> MHRFRVCALGAAFCVARRWRSGGGPGDRRVRTDWYRCYPSLMEEKDRDMYHCYYPYLFDHGDKMSLYPKIPDNPREWQVEQLQTTYDAIREDKYDAFVRLRAKFPELYQDTYAWDNPPPFGEFNMFYSVRFGMIGVKAFTCKDYDDLGNQFDCTAFWFPDNQIVKHSTRNGDVGTDKVYVGAMNVPVEFHKPHVAAFYKAAGVPVKHVSAGFPVTPDAYAPVGTKLDVRHFKPGQEVTITFQNTDYGYQGVMFRHGFDGGYVWLGDSKWQRRPGCMGAEGQKRIY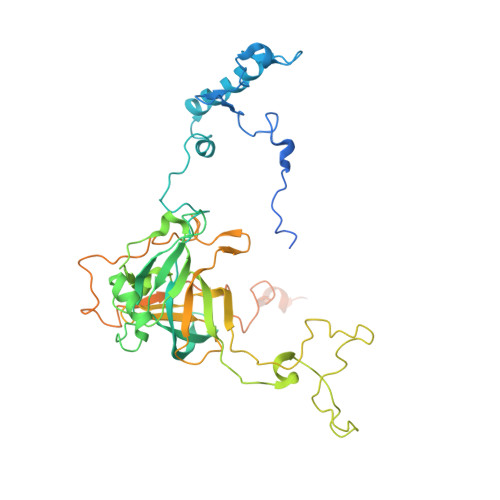PGHRMAGQTGASAETYDGVPVWRIDYKNSLIYLPTLIDADVGTYVKFRDTINTKGYTLWNEHRGTPPFPTFIPSEEEDLSKLATDEGQLTSPPLYMYFRDEFAAAQLVTQADVEDAKSAKPATAAPKKKVYDLKKYTEARKKYRKNLQKARKYKLMGVRTRAHEKQQEARRAKILKYKRVKT> MKYQSQSIALVYFAVALGLFAIQVSGGLLLGWIYVSPNFLSEILPFNIVRMLHTNSLIVWLLLGFMGAAYFVIPEESEREIHSPLLAYLQLAIMVLGTLGVVVTYLFNLFEGNWLLGKEGREFLEQPVWVKMGIVVAALIFMYNISMTVLQGRKTAITNVLLLGLWGLTLLFLFAFYNPSNLALDKMYWWYVVHLWVEGTWELVMASVLAFLMLKLTGVDRE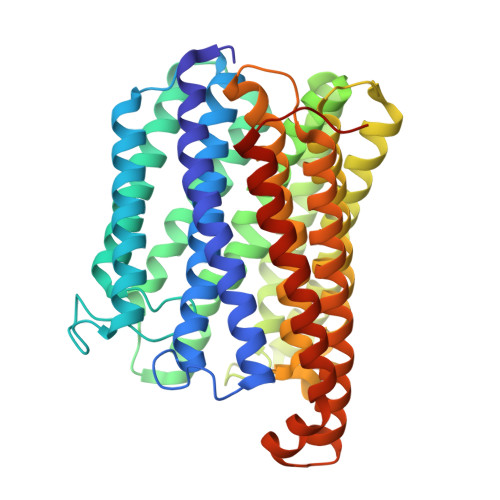IIEKWLYLIVATALFSGILGTGHHYFWIGTPGYWQWIGSIFSALEVVPFFGMMAFAFVMVWKGRKDHPNKAALLWSLGCATLAFFGAGVWGFLHTLHGINYYTHGTQITAAHGHLAFFGAYVSLNLAIFSYAFPILRKRDPYNQVLNMASFWLMAGGMTFMTFVLTFAGTVQTHAQRVQGDYFMDVQDAITIFYWMRFGSGIAVVLGALLFIYAVAVPRKEIISPSDKQPVAAE> MLICNFLMYSNFSRIYWFDFNGTVNENLPLNYNVLKICRNEINKLEKLNENNLGTQKNPIKLNLSFEDKHYNTNNLVLDLNSYETFNSKNFISSIFDKTFESLNTVLMAPIYSFLEFKLKLSSTKINTNHYYVINGKLYITYNDSFKLFTTINDYFNDLNELSNTKLFFLYRSFNIYNIKLNSLVDFVFLKLILFIHLLYLKSTNYNRFDYRLKQTDWGFYINNNSNYIQNIFSGLKYIWRGLRFWIIGLLLGLSSIYYLMYVRLLPFNKIIFAWILVAMFLYWLLSGFVFFVKKYQYSKFTAAIQRFWKRTYIIFWVIEAGTFSVFFYLTLNASSEPVYMYDQIKIYKTHLFSWRWFLIKLLPSVSIILLGYYLQLTLKWNLFNKQNTIVLLITLLLLYILWLEFYQFYHILSFYGNINW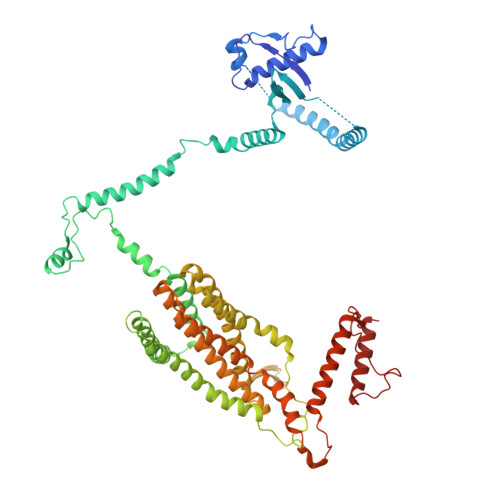AFDYDEYIWTLELDTRRTRLANNYIAICLFAKFWHFVFIFLFWVFFVLRINELGRIRYPLLVANVQNFIIIYIMSWAYMYPWLKFIFRKYLDVPYYWFYLNGRELGIRVFFTDLKLFFYGITNRLFDFNPSSIKFEKYPFYYWINSSQLTEFNQYRKFVIRDSIIYSLNNYII> GPVEDAITAAIGRVADTVGTGPTNSEAIPALTAAETGHTSQVVPGDTMQTRHVKNYHSRSESTIENFLCRSACVYFTEYENSGAKRYAEWVLTPRQAAQLRRKLEFFTYVRFDLELTFVITSTQQPSTTQNQDAQILTHQIMYVPPGGPVPDKVDSYVWQTSTNPSVFWTEGNAPPRMSIPFLSIGNAYSNFYDGWSEFSRNGVYGINTLNNMGTLYARHVNAGSTGPIKSTIRIYFKPKHVKAWIPRPPRLCQYEKAKNVNFQPSGVTTTRQSITTMTNTGAF;> SPTVEECGYSDRARSITLGNSTITTQECANVVVGYGVWPDYLKDSEATAEDQPTQPDVATCRFYTLDSVQWQKTSPGWWWKLPDALSNLGLFGQNMQYHYLGRTGYTVHVQCNASKFHQGCLLVVCVPEAEMGCATLDNTPSSAELLGGDSAKEFADKPVASGSNKLVQRVVYNAGMGVGVGNLTIFPHQWINLRTNNSATIVMPYTNS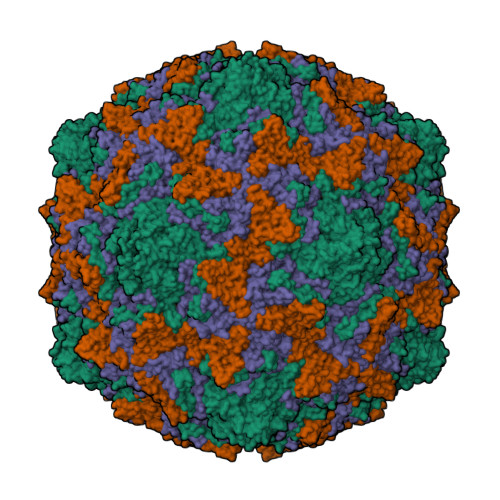VPMDNMFRHNNVTLMVIPFVPLDYCPGSTTYVPITVTIAPMCAEYNGLRLAGHQ;> GLPTMNTPGSCQFLTSDDFQSPSAMPQYDVTPEMRIPGEVKNLMEIAEVDSVVPVQNVGEKVNSMEAYQIPVRSNEGSGTQVFGFPLQPGYSSVFSRTLLGEILNYYTHWSGSIKLTFMFCGSAMATGKFLLAYSPPGAGAPTKRVDAMLGTHVVWDVGLQSSCVLCIPWISQTHYRYVTSDEYTAGGFITCWYQTNIVVPADAQSSCYIMCFVSACNDFSVRLLKDTPFISQQNFFQ;> MGAQVSTQKTGAHETGLNASGNSIIHYTNINYYKDAASNSANRQDFTQDPGKFTEPVKDIMIKSLPALN Here, we characterize the structure and function of a thermophilic dNDT, the protein from Chroococcidiopsis thermalis (CtNDT). Nucleoside 2′-deoxyribosyltransferase (dNDT) enzymes catalyze transglycosylation via a covalent 2′-deoxyribosylated enzyme intermediate with retention of configuration, having applications in the biocatalytic synthesis of 2′-deoxynucleoside analogues in a single step. The reaction catalyzed by dNDT proceeds via a ping-pong mechanism, with the formation of a 2′-deoxyribosyl-enzyme intermediate covalently linked to an active-site glutamate.13 Transglycosylation occurs in a stereospecific manner, preserving the anomeric carbon in the β configuration in the newly formed 2′-deoxyribonucleoside. As with other NDT enzymes, the active site of CtNDT is formed by residues from two monomers, and therefore, it is only fully formed in the dimer/tetramer.

Although dNDT enzymes are selective for 2′-deoxyribonucleosides, molecular detail underlying this preference is lacking. We therefore determined the structure of a ribosylated enzyme intermediate by cocrystallization of wild-type CtNDT in the presence of Ado. Residues D82 and N118 are in close proximity to the 5′-OH of the intermediate (3.3 and 3.5 Å, respectively). D62 is in very close proximity (2.6 Å) from 2′-OH and to 3′-OH (3.2 Å), and the proximity to 2′-OH (absent in 2′-deoxyribonucleosides) can lead to less optimal positioning of this intermediate for nucleophilic attack by the incoming nucleobase 2. An important observation is the positioning of Y7, likely polarizing the –COO– side chain of E88. Y7 does not directly interact with ligands, nor is it at a close enough distance to clash with a potential 2′-OH in the ribonucleoside ligand. One possibility is that Y7 restricts the movement of catalytic E88, but this optimal positioning for 2′-deoxyribonucleosides results in clashes between D62 and the 2′-OH of ribonucleoside substrates, leading to a reduced catalytic efficiency with these substrates. However, an over 100-fold difference in kcat between 2′-dGuo and Guo (6.9 ± 0.7 s–1 at 45 °C for 2′-dGuo and 0.06 ± 0.01 s–1 at 65 °C for Guo) indicates that nucleobase transfer is unfavorable with ribonucleoside substrates.

>[4x]MKRKIIYLASPYGFSQQQKTLLLPPIVRALEALGIEVWEPFARNNQIDFSQADWAYRVAQADLQDVKNCDGIFAVVNGTPPDEGVMVELGMAIALNKAIFLFRDDFRRCSDNERYPLNLMLFAGLPEIGWENYYYTSVDEIQSHDKALYKWLTG> GSTELTPDQQTLLHFIMDSYNKQRMPQEITNKILKEEFSAEENFLILTEMATNHVQVLVEFTKKLPGFQTLDHEDQIALLKGSAVEAMFLRSAEIFNKKLPSGHSDLLEERIRNSGISDEYITPMFSFYKSIGELKMTQEEYALLTAIVILSPDRQYIKDREAVEKLQEPLLDV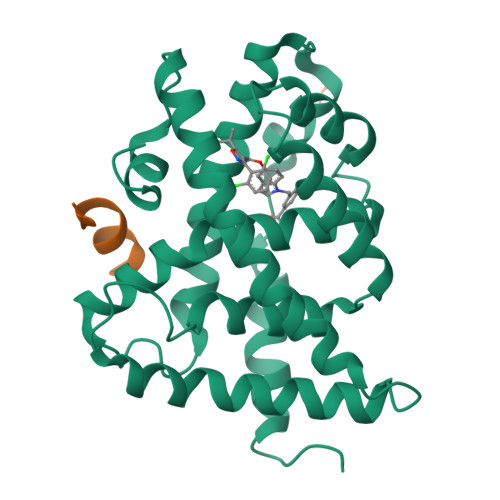LQKLCKIHQPENPQHFAELLGRLTELRTFNHHHAEMLMSWRVNDHKFTPLLEEIWDVQ;> KESKDHQLLRYLLDKDEKDLR>[4x]MEKDLQLRVNEKLDVENILKDLDKYTPKRRGWTWRQPAENLQMGPFIYKDASTPLENSVALPSAKYFGDIDPQPLPVITTEIASGRFEDDIRRMRMAAWHGADHIMVIRTAGQSHYDGLIEGTPQGIGGVPITRKQVRAQRKALDLIEEEVGRPINYHSYVSGVAGPDIAVMFAEEGVNGAHQDPQYNVLYRNINMIRSFIDACESKTIMAWADMAQIDGAHNANATAREAWKVMPELMVQHALNSIFSLKVGMKKSNICLSTVPPTAPPAPSMYLDLPYAVALREMFEGYRMRAQMNTKYMEASTREATVTHVLNLLISKLTRADIQSTITPDEGRNVPWHIYNIEACDTAKQALIGMDGLMDMVQLKREGVLGDTVRELKERAVLFMEEIIEAGGYFNAVEQGFFVDSGYYPERNGDGIARQINGGIGAGTVFERDEDYMAPVTAHF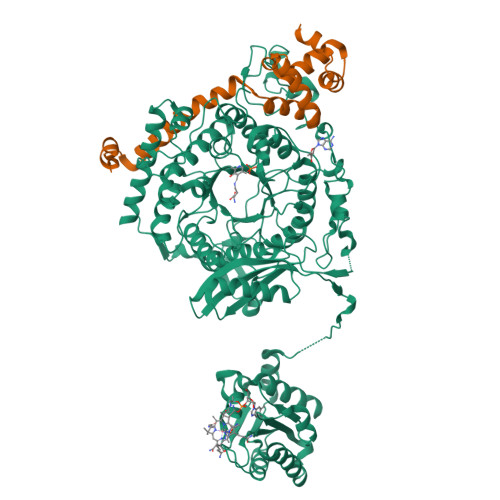GYNNVKQYDEALVSEPSKLIDGCTLEVPEKIVYIDELDENDNVNVRMEETKEFRHSSMIKPEVEWQADGTVLLTMFLPTSKRVAEFAAIEFAKKMNLEEVEVINREVMQEAEGTRIELKGRVPFSIDINSLVIPPEPEILSEDEIREDIEKTPLKIVAATVGEDEHSVGLREVIDIKHGGIEKYGVEVHYLGTSVPVEKLVDAAIELKADAILASTIISHDDIHYKNMKRIHELAVEKGIRDKIMIGCGGTQVTPEVAVKQGVDAGFGRGSKGIHVATFLVKKRREMREGKSEDPNSSSVDKLAAALEHHHHHH;>[4x]MKRADDFQQRRAHLANLSDEELQTRFWEMAEKIVDPLLDLGKKNTTPSIERSVLLRMGFSSLEAKAIVDKTMDRGLMGKGAGHIVYKIAKEKNISVREAGLALSEGKYWDDAIQIFKGGVK>SSSSTASASAKKIIVKHVTVIGGGLMGAGIAQVAAATGHTVVLVDQTEDILAKSKKGIEESLRKVAKKKFAENPKAGDEFVEKTLSTIATSTDAASVVHSTDLVVEAIVENLKVKNELFKRLDKRAAEHTIFASNTSSLQITSIANATTRQDR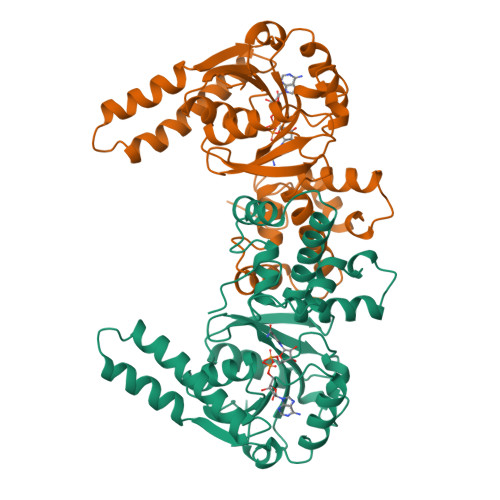FAGLHFFNPVPVMKLVEVIKTPMTSQKTFESLVDFSKALGKHPVSCKDTPGFIVNRLLVPYLMEAIRLYERGDASKEDIDTAMKLGAGYPMGPFELLDYVGLDTTKFIVDGWHEMDAENPLHQPSPSLNKLVAENKFGKKTGEGFYKYKHHHHHH[2x]> EVDKRREINNEHPLLMMPLYANGEEFNQGKYTFWGGDTLTGKWENIPDDLKPYTVIQLHPDDLPKRDGAARDFYEHMLEEAAKYVNPKTGKNEPIPVILTVYTAGNMPYHTSAHWLSTSWIDKMYQKYPNLHGIFSTASYWIWANDIENKAADYLKVSAKNGGYFIWAEQNSGSAIEKAFGKNGKIAFQKSVDKYWKNLIFMFKNTPAAEGNDSTTESYMKGLWLSNHTYQWGGLMDTWKWYET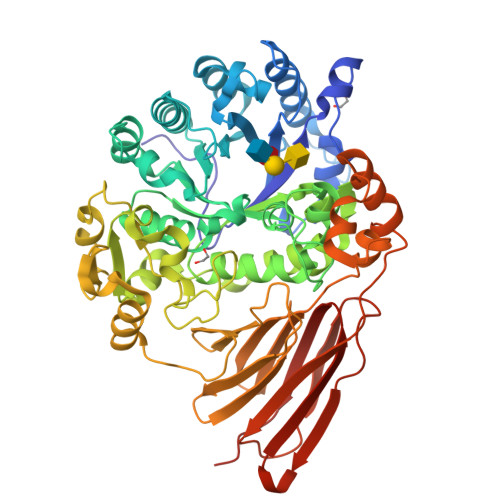GKWKLFASGNIGKSQGDRQWLTEPESMLGEEALGVYLNGGVVYNFEHPAYTYGVNNKESLLFSEVIKEFFRYVIAHPAPSKEKVLEDTKVFIHGDYSNKGNGKFFVNVNTDREQTPLYMTGRYNVIPAIPGVLKTDKLKESVSSSRIQIKEITSPEFSSTQARKEYLNKLYPMNYEGDIFAQKLDNRWFVYNYKVNENVKQTGKLKFNSLEMNVEFEPHTYGIFERISNGLKVNLNNFRTNKDSLWSNAQDANQAKKLPQLTKKGAIKWIEEHYIKDTQFGEKRVTKIVLRGIDKLPTIHSLSGTNNSYDQPSLNFDQKNHMVTITINSNGNLEFELHFLEHTRAPPPPPLRSGC> MEGGKLQSTFVFEEIGRRLKDIGPEVVKKVNAVFEWHITKGGNIGAKWTIDLKSGSGKVYQGPAKGAADTTIILSDEDFMEVCLGKLDPQKAFFSGRLKARGNIMLSQKLQMILK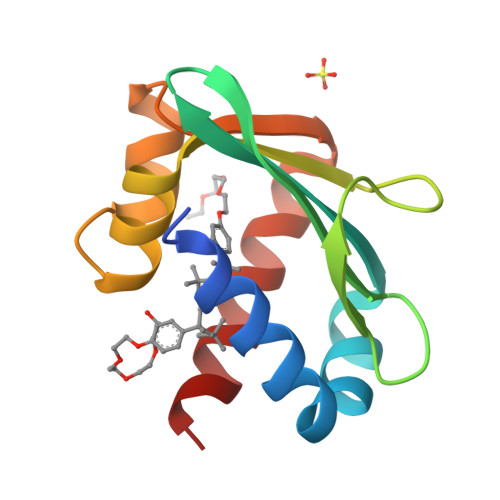DYAKL>[2x]GPMRCGVVPFHGTSEVWMVPSKESGWILPKGGLDVQDGGDWETCVRREAREEGGFTLGPVEYLGTFGDIVWYKGTVTHKSDPTDPEVKARGPAKHFTISDARGYLTGYGKKK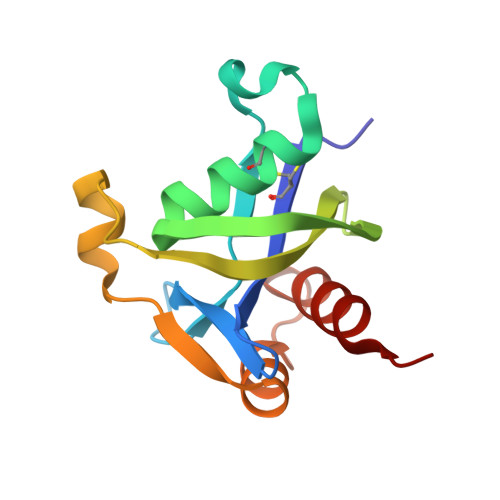DAMLEALNAATRGS>[2x]MPNIKIFSGSSHQDLSQKIADRLG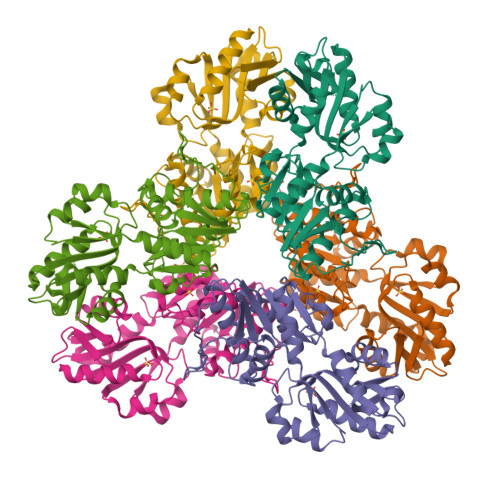LELGKVVTKKFSNQETCVEIGESVRGEDVYIVQSGCGEINDNLMELLIMINACKIASASRVTTVIPCFPYARQDKKDKSRAPISAKLVANMLSVAGADHIITMDLHASQIQGFFDIPVDNLYAEPAVLKWIRENISEWRNCTIVSPDAGGAKRVTSIADRLNVDFALIHKERKKANEVDRMVLVGDVKDRVAILVDDMADTCGTICHAADKLLSAGATRVYAILTHGIFSGPAISRINNACFEAVVVTNTIPQEDKMKHCSKIQVIDISMILAEAIRRTHNGESVSYLFSHVPLLEHHHHHH>IDPFTMSDLPCPPTNAERLHEFHRAIGAATPERPTPPPPELLRLRQTLLDEASAEVRAEIDHLLARQAAGEALSAGDLAPLAHELADLLYVTYGALDQLGIDADAVFAEVHRANLSKASGPRRADGKQLKPEGWRPADVRGVIERLQHAPA[4x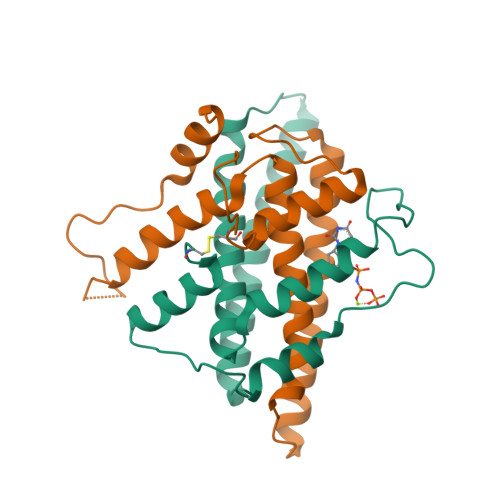]> GPPSRVIHIRKLPIDV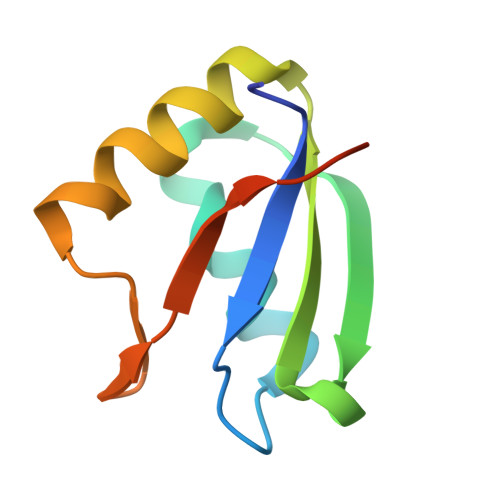TEGEVISLGLPFGKVTNLLMLKGKNQAFIEMNTEEAANTMVNYYTSVTPVLRGQPIYIQFSNHKELKTDS>MGSSHHHHHHHHLEVLFQGPHMMKPAKPLPKEMEEFVQSSGENGIVVFSLGSMISNMSEESANMIASALAQIPQKVLWRFDGKKPNTLGSNTRLYKWLPQNDLLGHPKTKAFITHGGTNGIYEAIYHGIPMVGIPLFADQHDNIAHMKAKGAALSVDIRTMSSRDLLN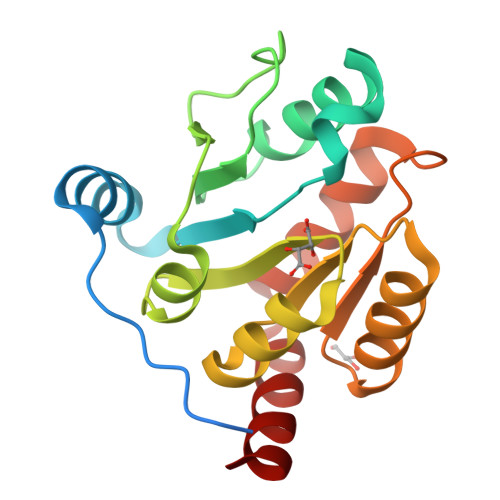ALKSVINDPVYKENVMKLSRIHH[4x]> GSHELLSKEEEEAKAKADKIKLALEKLKEAKVKKLVVKVHMDDSSTKSLMVDERQLARDVLDNLFEKTHCDCNVDWCLYEIYPELQIERVFEDHENVVEVLSDWTRDTENKVLFLEKEERYAVFKNPQNFYLDNKGKKENKETNEKMNAKNKEYLLEESFCGTSIIVPELEGALYLKEDGKKSWKRRYFLLRASGIYYVPKGKTKTSRDLACFIQFENVNIYYGIQCKMKYKAPTDHCFVLKHPQIQKESQYIKYL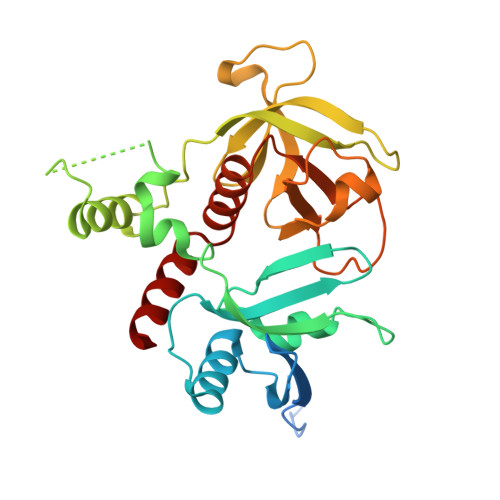CCDDARTLSQWVMGIRIAKYGKTLYDNYQRAVARA AGDC1 and PPP2 fit in none of these categories as both enzymes neither display cofactors bound to their active sites nor require the styrene motif or ATP hydrolysis. Instead, they act on the carboxyl-group directly attached to the aromatic ring. Intriguingly, these enzymes’ catalytic mechanism is a new type of decarboxylation mechanism combining acid–base catalysis by a His-Asp dyad with a sophisticated web of hydrogen bonds and a double tryptophan twisting clamp. The trimers of AGDC1 and PPP2 in the crystal structures represent the functional biological unit, evidenced by the size exclusion chromatography data and the extensive intermonomer buried surfaces and interactions.

Purified AGDC1 crystallized without any added ligands (apo-enzyme), except potassium from the crystallization solution, or with the substrate analog 4-nitrocatechol (4NC) in the presence of cobalt (4NC/Co2+ complex). Apo-AGDC1 crystallized with nine molecules in the AU, in the space group R3, forming a trimer of trimers. AGDC1 crystal structures were solved by molecular replacement, using the PPP2 4NC complex structure as a search probe. They were refined to 1.9 and 1.5 Å resolution for the apo-enzyme and 4NC/Co2+ complex structures, respectively. Surprisingly, the active site in the apo-structure has the same geometry as the 4NC complex structures. Here, however, several ordered water molecules occupy the space of 4NC. Although the exact geometry varies between the nine protein chains present in the asymmetric unit, active site residues R39, H86, W61, T60, Y150, Y146, and Q192 are involved in hydrogen-bond interactions with the ordered water molecules. In the apo-structure, which lacked cobalt in the crystallization buffer, H14 and E49 interact directly via a hydrogen bond. In all crystal structures, the center of the AGDC1 trimer contains a potassium ion. All structures contain a central metal-binding site, formed by three equivalent glutamate residues (E88), one from each monomer, which coordinate the metal with side chain and carbonyl oxygen interactions in a distorted octahedron. The organizational role of potassium may also explain the high similarity in the active sites of the apo-enzyme and the 4NC complex structures, both liganded with potassium present in crystallization conditions.

>MTTSYEPWPQLYSHLNGTNEEVLDRMKVAELCKGWSVYRDASEWANFKEMFTPDANIWTTWSGAQTIDSFIQISKDGKDKGAFIMHRECGTLVDLNPKTQRAIGKMKTTITQRFEYEGVPFDIDCDNYFIFFCLKDSNGDWKARWYKVFYVKDKFVPVGVPTAENMEKLAKLFSKENLEQYPWGYQYLAVAQANLGYPIDKKLPTWKNELYHTMYDAMKEWMEGKEIDLHW[9x]>HMTMEQFLTSLDMIRSGCAPKFKLKTEDLDRLRVGDFNFPPSQDLMCYTKCVALMAGTVNKKGEFNAPKALAQLPHLVPPEMMEMSRKSVEACRDTHKQFKESCERVYQTAKCFSENA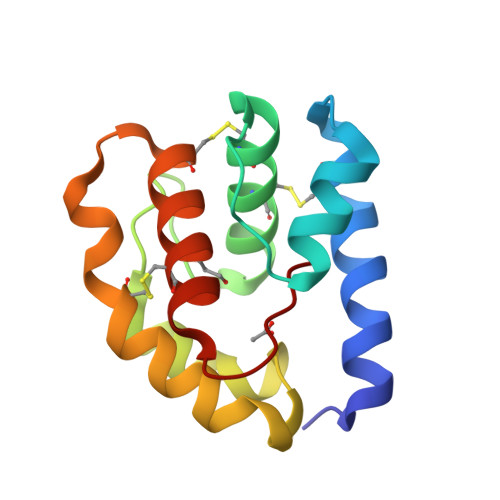DGQFMWP[2x]> MSDEWEQLTVELRKIPRGTEAAPQYLRHLMKMFVADFETAVSKRFDVKFWNKLKSMMDEITKAMENDR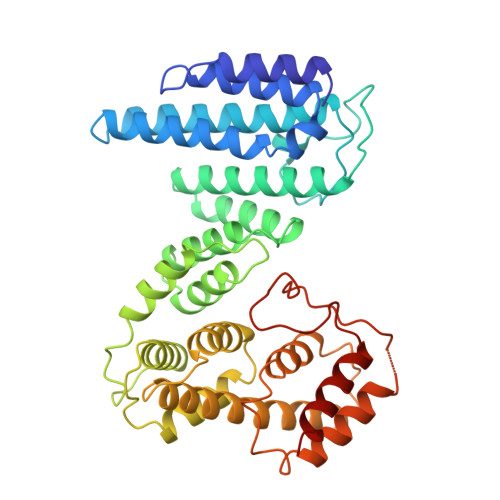LVNHNVQNLAIGFLTDLSLLVHYHYEIPNYGNDISKQLTWTPDVFLNRKPIKSKKNSRVFMAYVLLRMGDLMRYKENYPKAQEYYEQSCRINPADGAVWNQLGLISSLGAKNLESVYFHTRALHATMEFPTASGGLTNIFKNFANRDISRPMPIKDLYLSCLGRIHFLLEIEDSSVHLQKIGEEAATSKEMIVPLMSVYKHLEDGTELEQRAVEYVKTIWCTAYRSLLKTLDDYKEESKKLADVPHLLHILALLLCAPKLLRGIEDQTEDEVTSICEWLLCANCDEKIKDSDAFGYFHCLQRIQYPLTRTQLAQKLVEIEDEDESKD> MGMIQ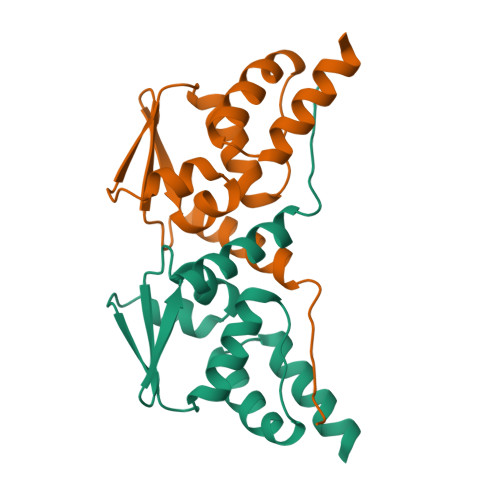LQNPSHPTGLLCKANQMRLAGTLCDVVIMVDSQEFHAHRTVLACTSKMFEILFHRNSQHYTLDFLSPKTFQQILEYAYTATLQAKAEDLDDLLYAAEILEIEYLEEQCLKMLETIQ The vacuolar-type H+-ATPases (V-ATPases), which localize to the plasma membrane, endosomes, and membrane-bound vesicles, are ATP-driven proton pumps which regulate intracellular pH homeostasis. V-ATPase is a rotary machine conserved from yeast to mammals. The V1 domain, containing sixteen subunits (A3B3CDE3FG3H), catalyzes the hydrolysis of ATP by the A3B3 heterohexamer to trigger the V1–Vo torque transmission via subunits DF. In this manuscript, we discovered that mEAK7, a lysosomal surface-anchored protein, can bind the V1 domain of intact V-ATPase and may function as an inhibitor of V-ATPase.

Since the yield of endogenous V-ATPase from HEK293 cells is low, we employed the endogenously purified V-ATPase from bovine brain to perform all in vitro assays. The mEAK7 binding sites are highly conserved in these two species. To confirm that bovine V-ATPase can be a competent substitute for human V-ATPase in these experiments, we purified human mEAK7 from E. coli and collected the cryo-EM data from a mixture of homo sapiens mEAK7 and bos taurus V-ATPase (hsmEAK7-btV-ATPase complex) at 10:1 molar ratio. The structural analysis showed that human mEAK7 could form a complex with bovine V-ATPase similar to human V-ATPase.

> MSGKDRIEIFPSRMAQTIMKARLKGAQTGRNLLKKKSDALTLRFRQILKKIIETKMLMGEVMREAAFSLAEAKFTAGDFSTTVIQNVNKAQVKIRAKKDNVAGVTLPVFEHYHEGTDSYELTGLARGGEQLAKLKRNYAKAVELLVELASLQTSFVTLDEAIKITNRRVNAIEHVIIPRIERTLAYIITELDEREREEFYRLKKIQEKKKILKEKSDKDLEQRRAAGEVIEPANLLAEEKDEDLLFE;>[3x]MDFSKLPKIRDEDKESTFGYVHGVSGPVVTACDMAGAAMYELVRVGHSELVGEIIRLEGDMATIQVYEETSGVSVGDPVLRTGKPLSVELGPGIMGAIFDGIQRPLSDISSQTQSIYIPRGVNVSALSRDVKWDFTPCKNLRVGSHITGGDIYGIVNENSLIKHKIMLPPRNRGTVTYIAPPGNYDTSDVVLELEFEGIKEKFSMVQVWPVRQVRPVTEKLPANHPLLTGQRVLDALFPCVQGGTTAIPGAFGCGKTVISQSLSKYSNSDVIIYVGCGERGNEMSEVLRDFPELTMEVDGKVESIMKRTALVANTSNMPVAAREASIYTGITLSEYFRDMGYHVSMMADSTSRWAEALREISGRLAEMPADSGYPAYLGARLASFYERAGRVKCLGNPEREGSVSIVGAVSPPGGDFSDPVTSATLGIVQVFWGLDKKLAQRKHFPSVNWLISYSKYMRALDEYYDKHFTEFVPLRTKAKEILQEEEDLAEIVQLVGKASLAETDKITLEVAKLIKDDFLQQNGYTPYDRFCPFYKTVGMLSNMIAFYDMARRAVETTAQSDNKITWSIIREHMGEILYKLSSMKFKDPVKDGEAKIKADYAQLLEDMQNAFRSLED;>[3x]MALRAMRGIVNGAAPELPVPTSGPLAGSREQALAVSRNYLSQPRLTYKTVSGVNGPLVILDHVKFPRYAEIVHLTLPDGTKRSGQVLEVSGSKAVVQVFEGTSGIDAKKTSCEFTGDILRTPVSEDMLGRVFNGSGKPIDRGPVVLAEDFLDIMGQPINPQCRIYPEEMIQTGISAIDGMNSIARGQKIPIFSAAGLPHNEIAAQICRQAGLVKKSKDVVDYSEENFAIVFAAMGVNMETARFFKSDFEENGSMDNVCLFLNLANDPTIERIITPRLALTTAEFLAYQCEKHVLVILTDMSSYAEALREVSAAREEVPGRRGFPGYMYTDLATIYERAGRVEGRNGSITQIPILTMPNDDITHPIPDLTGYITEGQIYVDRQLHNRQIYPPINVLPSLSRLMKSAIGEGMTRKDHADVSNQLYACYAIGKDVQAMKAVVGEEALTSDDLLYLEFLQKFERNFIAQGPYENRTVYETLDIGWQLLRIFPKEMLKRIPQSTLSEFYPRDSAKH;> MGHHHHHHGNSRSRVGRSFCSQFLPEEQAEIDQLFDALSSDKNSPNVSSKSFSLKALQNHVGEALPPEMVTRLYDGMRRVDLTGKAKGPSENVSQEQFTASMSHLLKGNSEEKSLMIMKMISATEGPVKAREVQKFTEDLVGSVVHVLSHRQELRGWTGKEAPGPNPRVQVLAAQLLSDMKLQDGKRLLGPQWLDYDCDRAVIEDWVFRVPHVAIFLSVVICKGFLVLCSSLDLTTLVPERQVDQGRGFESILDVLSVMYINAQLPREQRHRWRLLFSSELHGHSFSQLCGHITHRGPCVAVLEDHDKHVFGGFASCSWEVKPQFQGDNRCFLFSICPSMAVYTHTGYNDHYMYLNHGQQTIPNGLGMGGQHNYFGLWVDVDFGKGHSRAKPTCTTYNSPQLSAQENFQFDKMEVWAVGDPSEEQLAKGNKSILDADPEAQALLEISGHSRHSEGLREVPDDE;>[3x]MALSDADVQKQIKHMMAFIEQEANEKAEEIDAKAEEEFNIEKGRLVQTQRLKIMEYYEKKEKQIEQQKKIQMSNLMNQARLKVLRARDDLITDLLNEAKQRLSKVVKDTTRYQVLLDGLVLQGLYQLLEPRMIVRCRKQDFPLVKAAVQKAIPVYKVATKRDVDVQIDQEAYLPEEIAGGVEIYNGDRKIKVSNTLESRLDLIAQQMMPEVRGALFGANANRKFLD;>MASQSQGIQQLLQAEKRAAEKVADARKRKARRLKQAKEEAQMEVDQYRREREQEFQSKQQAAMGSQGNLSAEVEQATRRQVQGMQSSQQRNRERVLAQLLGMVCDVRPQVHPNYRIAA[3x]>MSAEHVLTMLNEHEVKFVDLRFTDTKGKEQHVTIPAHQVNAEFFEEGKMFDGSSIGGWKGINESDMVLMPDASTAVIDPFFADSTLIIRCDILEPGTLQGYDRDPRSIAKRAEDYLRSTGIADTVLFGPEPEFFLFDDIRFGSSISGSHVAIDDIEGAWNSSTQYEGGNKGHRPAVKGGYFPVPPVDSAQDIRSEMCLVMEQMGLVVEAHHHEVATAGQNEVATRFNTMTKKADEIQIYKYVVHNVAHRFGKTATFMPKPMFGDNGSGMHCHMSLSKNGVNLFAGDKYAGLSEQALYYIGGVIKHAKAINALANPTTNSYKRLVPGYEAPVMLAYSARNRSASIRIPVVSSPKARRIEVRFPDPAANP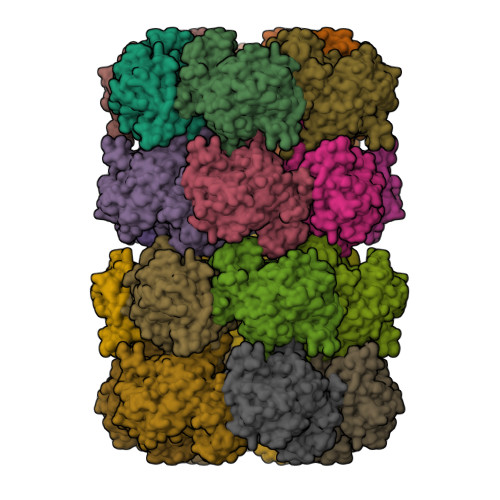YLCFAALLMAGLDGIKNKIHPGEAMDKNLYDLPPEEAKEIPQVAGSLEEALNELDLDREFLKAGGVFTDEAIDAYIALRREEDDRVRMTPHPVEFELYYSV[24x]>[4x]DENASAAEQVNKTIIGIDPGSGIMSLTDKAMKDYDLNDWTLISASSAAMTATLKKSYDRKKPIIITGWTPHWMFSRYKLKYLDDPKQSYGSAEEIHTITRKGFSKEQPNAAKLLSQFKWTQDEMGEIMIKVEEGEKPAKVAAEYVNKHKDQIAEWTKGVQKVKGDKINLAYVAWDSEIASTNVIGKVL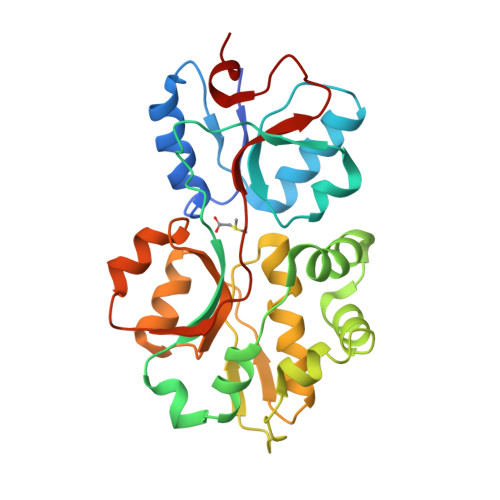EDLGYEVTLTQVEAGPMWTAIATGSADASLSAWLPNTHKAYAAKYKGKYDDIGTSMTGVKMGLVVPQYMKNVNSIEDLKK> AFRDDIIAGFANTRWLGLTIFEHTWSEAENTGYVSFIARFSEQGKNGA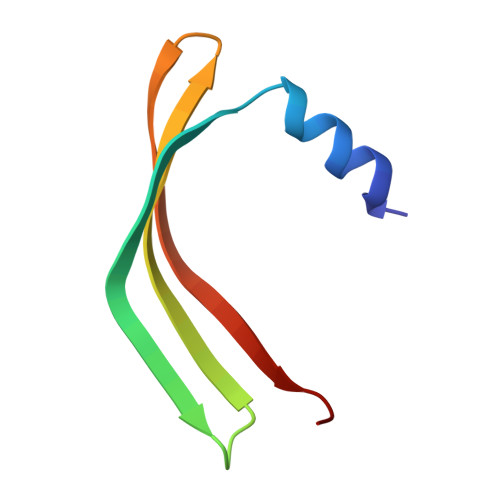IIERSRFIKENG>GMLRISQEALTFDDVLLIPGYSEVLPKDVSLKTRLTRGIELNIPLVSAAMDTVTEARLAIAMAQEGGIGIIHKNMGIEQQAAEVRKVKKHETAIVRDPVTVTPSTKIIELLQMAREYGFSGFPVVEQGELVGIVTGRDLRVKPNAGDTVAAIMTPKDKLVTAREGTPLEEMKAKLYENRIEKMLVVDENFYLRGLVTFRDIEKAKTYPLASKDEQGRLRVGAAVGTGADTGERVAALVAAGVDVVVVDTAHGHSKGVIERVRWVKQTFPDVQVIGGNIATAEAAKALAEAGADAVKVGIGPGSICTTRIVAGVGVPQISAIANVAAALEGTGVPLIADGGIRFSGDLAKAMVAGAYCVMMGSMFAGTEEAPGEIELFQGRSYKSYRGMGSLGAMSGSQGSSDRYFQDASAGAEKLVPEGIEGRVPYKGALSAIVHQLMGGLRAAMGYTGSADIQQM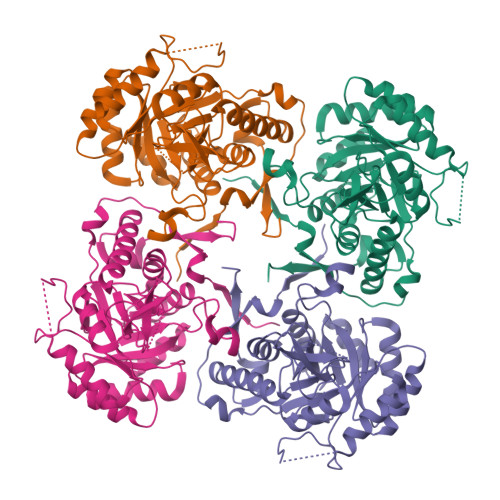RTQPQFVRITGAGMAESHVHDVQITKEAPNYRVG[4x]>[2x]MGSSHHHHHHSSGLVGRPSHMMTHPHRPVRGRSPRTLVLACVTALAVATTGFAVAETRDGERAAAADGRQAFDFTEGNSALEVIYPRVGPAVRKHINQVAMDGTLVLRVSALMESSWFDATAPYHPTAVGIHSDLGRRPASEATQKNLNTAMLYSTYRVMQSLMPTYDAQWREMLTSVGLDPDDDSTDRTTPVGLGNAAGNAVVEKRENDGMNQLGNEGGQKYHQRPYSDYTGYKPVNTPYDIRNPSRWQPALVSTGNGIFTAQSFVTAQLGRAKPYSFADPKDLLVSKPRSSNHRNRAAYKRQAEEVLRASANLTDEQKLKAEFFN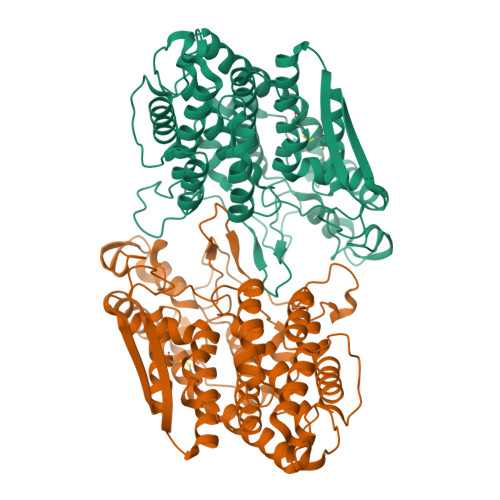DKLIFASGFMGEISDDLMEFIHSATASHIAGFDVMLASWYNKRKYDAPRPFTAIRYLYAGQKLRAWGGPGKGTVDDMPAEDWQSYLQVSDHPEYPSGSTAFCAAQAEVGKLVGGGDRTDIRYDVEKGGSYIEPGVTPAKDTSIRWTDWNEMVDDCAKSRVWGGVHFKAATEASKGLGAKVGESSYRYVQSHIEGKQVGSMR>MSAKDTADLSPLLEANRKWADECAAKDSTYFSKVAGSQAPEYLYIGCADSRVSPAQLFNMAPGEVFVQRNVGNLVSNKDLNCMSCLEYTVDHLKIKHILVCGHYNCGACKAGLVWHPKTAGVTNLWISDVREVRDKNAAKLHGLSADDAWDKMVELNVEAQVFNVCASPIVQAAWARGQPLSVH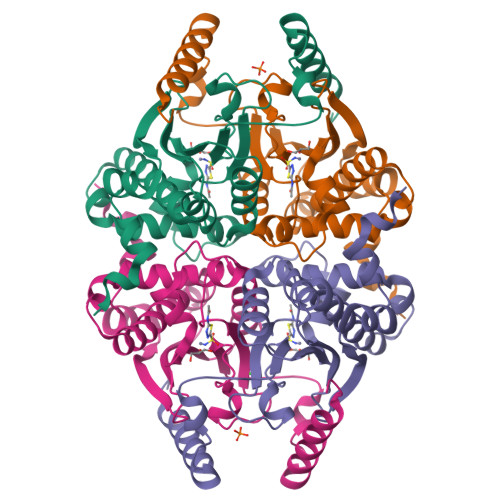GIVYTPGTGLVKELIKPITGMEDAGALLRADLKQHCFFSESLA[2x]> MNNIWWQTKGQGNVHLVLLHGWGLNAEVWRCIDEELSSHFTLHLVDLPGFGRSRGFGALSLADMAEAVLQQAPDKAIWLGWSLGGLVASQIALTHPERVRALVTVASSPCFSARDEWP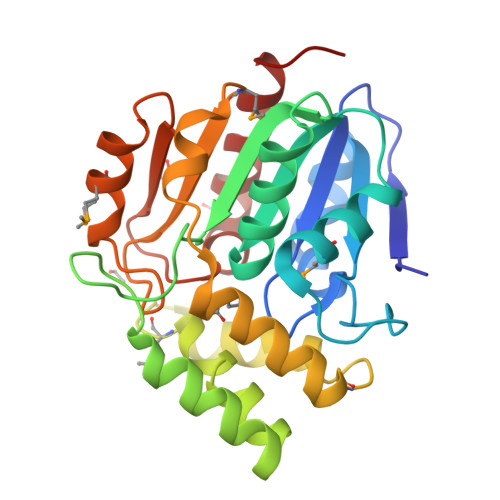GIKPDVLAGFQQQLSDDQQRTVERFLALQTMGTETARQDARALKKTVLALPMPEVDVLNGGLEILKTVDLRQPLQNVSMPFLRLYGYLDGLVPRKVVPMLDKLWPHSESYIFAKAAHAPFISHPAEFCHLLVALKQRVGS> DEEITCQENLPFTCGNTDALNSSSFSSDFIFGVASSAYQIEGTIGRGLNIWDGFTHRYPNKSGPDHGNGDTTCDSFSYWQKDIDVLDELNATGYRFSIAWSRIIPRGKRSRGVNEKGIDYYHGLISGLIKKGITPFVTLFHWDLPQTLQDEYEGFLDPQIIDDFKDYADLCFEEFGDSVKYWLTINQLYSVPTRGYGSALDAPGRCSPTVDPSCYAGNSSTEPYIVAHHQLLAHAKVVDLYRK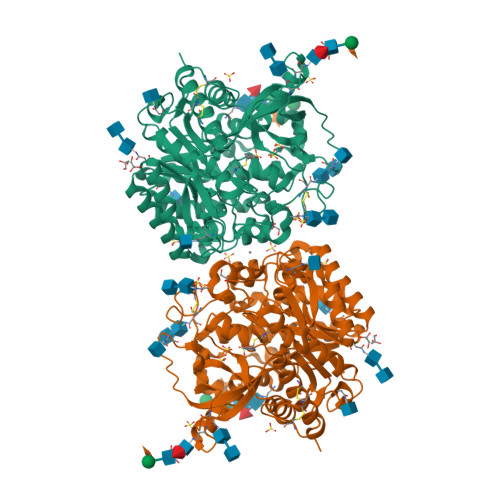NYTHQGGKIGPTMITRWFLPYNDTDRHSIAATERMKEFFLGWFMGPLTNGTYPQIMIDTVGERLPSFSPEESNLVKGSYDFLGLNYYFTQYAQPSPNPVNSTNHTAMMDAGAKLTYINASGHYIGPLFEKDKADSTDNIYYYPKGIYSVMDYFKNKYYNPLIYVTENGISTPGDENRNQSMLDYTRIDYLCSHLCFLNKVIKEKDVNVKGYLAWALGDNYEFNKGFTVRFGLSYIDWNNVTDRDLKKSGQWYQSFISP The novel enterotoxin of C. perfringens W5052 consists of two unlinked components: CPILE-a, which acts as an enzymatic ADP-ribosyltransferase (ART), and CPILE-b, a membrane binding and pore forming component. The structure of CPILE-a can be divided into two domains, N-terminal (amino acids 3–211) and C-terminal (amino acids 212–419). Even though they had a low sequence identity (29%), the structure of N-terminal and C-terminal domain are homologous (1.3 Å RMSD / 133 Cα atoms). We conducted detailed analysis of actin ADP-ribosylation by each CPILE-a and Ia against both α- and β/γ-actin. These characterizations show that newly found CPILE-a is a unique ART which has different structural and substrate recognition features from Ia.

Using mercury-soaked crystal data, the structure of CPILE-a was solved using SHELX against the single anomalous dispersion data set at 2.28 Å resolution. Using the triple Cys mutant structure as a template, the final structure of wild type CPILE-a was refined at 2.01 Å resolution. The CPILE-a crystal belongs to space group I222 and consists of one molecule in an asymmetric unit. There was a long loop at the junction between the N- and C-terminal domains. The overall structure of CPILE-a was similar to that of other type IV ARTs. Comparison to Ia, CPILE-a contained a flexible loop (A60-I67). The corresponding region in Ia (Y60-E65) forms an α-helix (loop I). Moreover, two protruding loops in CPILE-a were not seen in Ia: G262-S269 and E402-K408, which are considered to be crucial regions for the binding of actin. Thus, these two loops were named PT-I (G262-S269) and PT-II (E402-K408).

> GSMLDDNRPMDFAKDKNSATLWAKKRKQVWLNNLSKAESTSINNYIKNSSEINSYSIKKKFALDNYEGIETLNEDLKNISTAVKKSMLTKPLYVYYYEANDKFGFNQNLESSLDSNIIDEEAINNFAKKISDTNFIQDGFKDVTMTEPDINSKLPILVHLKLPTNTPAASYGNDEENLRVLIDQGYSLKATGLSIVTIKGKQYAKVDADLIKQLNFENDVISASQWGEENYAPWLKELTSNELRDINNYLGGGYTAINKYLLDGTIGENTSKEDLEEKISNISSALKKRKIPEDIITYRRMGPNEFGLDLNSPDYDFNKVENVSKFKEKWLGKTIPVKTFISTTVLSNNISAFAKRKLILRLHLPNGSNAAYVSVAEGYKNEYEVLIDHGYSYKIDNITEYYDESSLGGKTNKLIIDATLI> MTSKVYDPEQRKRMITGPQWWARCKQMNVLDSFINYYDSEKHAENAVIFLHGNATSSYLWRHVVPHIEPVARCIIPDLIGMGKSGKSGNGSYRLLDHYKYLTAWFELLNLPKKIIFVGHDWGAALAFHYAYEHQDRIKAIVHMESVVDVIESWDEWPDIEEDIALIKSEEGEKMVLENNFFVETVLPSKIMRKLEPEE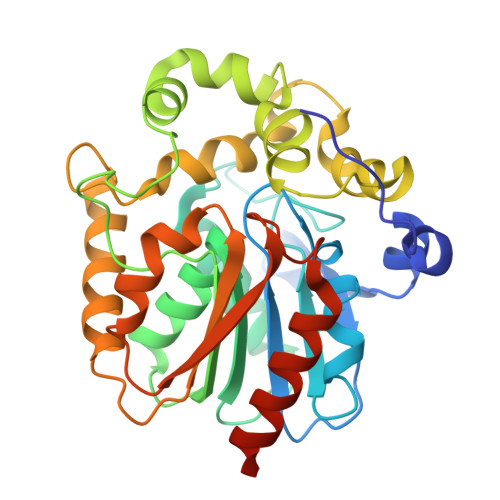FAAYLEPFKEKGEVRRPTLSWPREIPLVKGGKPDVVQIVRNYNAYLRASDDLPKLFIESDPGFFSNAIVEGAKKFPNTEFVKVKGLHFLQEDAPDEMGKYIKSFVERVLKNEQSGLEVLFQ>[2x]PLNKFPGFAKPGTEQYLLAKQLAKPKEKIPIIVGDYGPMWVYPTSTFDCVVADPRKGSKMYGLKSYIEYQLTPTNTNRSVNHRYKHFDWLYERLLVKFGSAIPIPSLPDKQVTGRFEEEFIKMRMERLQAWMTRMCRHPVISESEVFQQFLNFRDEKEWKTGKRKAERDELAGV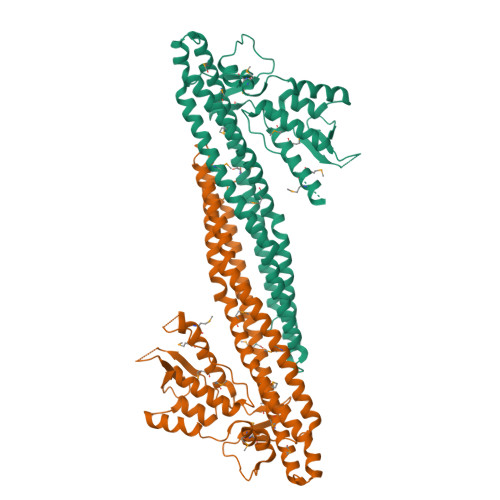MIFSTMEPEAPDLDLVEIEQKCEAVGKFTKAMDDGVKELLTVGQEHWKRCTGPLPKEYQKIGKALQSLATVFSSSGYQGETDLNDAITEAGKTYEEIASLVAEQPKKDLHFLMECNHEYKGFLGCFPDIIGTHKGAIEKVKESDKLVATSKITLQDKQNMVKRVSIMSYALQAEMNHFHSNRIYDYNSVIRLYLEQQVQFYETIAEKLRQALSRFPVM In Gram-negative bacteria, conjugation is mediated by a large transport apparatus—the conjugative type IV secretion system (T4SS)—produced by the donor cell and embedded in both its outer and inner membranes. The T4SS also elaborates a long extracellular filament—the conjugative pilus—that is essential for DNA transfer. Here we present a single-particle cryo-EM structure of a T4SS complex from the R388 plasmid that comprises all four sub-complexes: OMCC, stalk, arches and IMC. Three ATPases, VirB4 (also known as TrwK), VirB11 (also known as TrwD) and VirD4, power the system.

The IMC is 1.32 MDa in size and 295 Å in diameter. The IMC is composed of six protomers, each including one VirB3 (also known as TrwM), two VirB4, and the three N-terminal tails of VirB8 (hereafter referred to VirB8tails; VirB8 is also known as TrwG). Three of these protomers are occupied to a significant degree, whereas the occupancy of the three others is weaker. All protomers were related by an angle of 60°. The IMC is thus a hexameric structure with compositional heterogeneity (that is, variable occupancy of its constituent protomers) as defined by Huiskonen17, thereby limiting our ability to observe interactions and transitions in situ. The main component of the IMC is the AAA+ VirB4 ATPase, for which 12 subunits are present. In the IMC, six dimers of VirB4 come together to form a hexamer of dimers. One subunit (VirB4central) in each of the 6 dimers form a central hexamer with a diameter of 130 Å. The second subunit of the dimers (VirB4outside; structurally very similar to VirB4central) protrudes out (in cyan blue in Fig. 2). The arches (the composition and architecture of which were previously unknown) are composed of hexamers of homotrimeric units of VirB8peri, forming a 177 Å diameter ring around the stalk.

>MGAIESRKLLASETPVGQFIPYSHHVTDTIISTKNAEYLSVWKIDGRSHQSASEADVFQWIRELNNTLRGISSANLSLWTHIVRRRVYEYPDAEFDNVFCRQLDEKYRESFTGYNLMVNDLYLTVVYRPVSDKVLSFFAKRERETPDQKKHRQESCIKALEDINRTLGQSFKRYGAELLSVYEKGGHAFSAPLEFLARLVNGEHIPMPICRDRFSDYMAVNRPMFSKWGEVGELRSLTGLRRFGMLEIREYDDATEPGQLNVLLESDYEFVLTHSFSVLSRPAAKEYLQRHQKNLIDARDVATDQIEEIDEALNQLISGHFVMGEHHCTLTVYGETVQQVRDNLAHASAAMLDVAVLPKPVDLALEAGYWAQLPANWQWRPRPAPITSLNFLSFSPFHNFMSGKPTGNPWGPAVTILKTVSGTPLYFNFHASKEEEDATDKRLLGNTMLIGQSSSGKTVLLGFLLAQAQKFKPTIVAFDKDRGMEISIRAMGGRYLPLKTGEPSGFNPFQLPPTHANLIFLKQFVKKLAAAGGEVTHRDEEEIDQAITAMMSDSIDKSLRRLSLLLQFLPNPRSDDMDARPTVHARLVKWCEGGDYGWLFDNPTDALDLSTHQIYGFDITEFLDNPEARTPVMMYLLYRTESMIDGRRFMYVFDEFWKPLQDEYFEDLAKNKQKTIRKQNGIFVFATQEPSDALESNIAKTLIQQCATYIFLANPKADYEDYTQGFKLTDSEFELVRGLGEFSRRFLIKQGDQSALAEMNLGKFRTIVDGETVERDFDDELLVLSGTPDNAEIAESIIAEVGDDPAVWLPIFLDRVKAERSDV[2x];> MKPPQQQHEAFPLFKGATRLPTIWGVPMIPLMAMVMGVAVIALTVSIWWWALVPPLWFIMAQITKNDDKAFRIWWLWIDTKFRNRNKGFWGASSYSPANYRKRR;>[3x]MSKKQPKPVKAEQLKSYYEESRGLERDLIGEFVKSRKTAWRVATASGLFGLLGMVCGIVGFSQPAPAPLVLRVDNATGAVDVVTTLREHESSYGEVVDTYWLNQYVLNREAYDYNTIQMNYDTTALLSAPAVQQDYYKLFDGSNARDRVLGNKARITVRVRSIQPNGRGQATVRFTTQQHNSNGTVEAPQHQIATIGYTYIGAPMRSSDRLLNPLGFQVTSYRADPEILNN[4-({4-[(5-cyclopropyl-1H-pyrazol-3-yl)amino]-6-(methylamino)pyrimidin-2-yl}amino)phenyl]acetonitrile 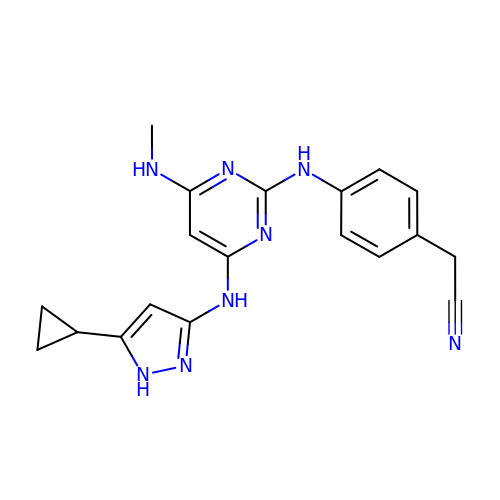| C19 H20 N8 | MFMSRHREFZCFSN-UHFFFAOYSA-N>[2x]GSHMRSRRVDVMDVMNRLILAMDLMNRDDALRVTGEVREYIDTVKIGYPLVLSEGMDIIAEFRKRFGCRIIADFAVADIPETNEKICRATFKAGADAIIVHGFPGADSVRACLNVAEEMGREVFLLTEMSHPGAEMFIQGAADEIARMGVDLGVKNYVGPSTRPERLSRLREIIGQDSFLISPGVGAQGG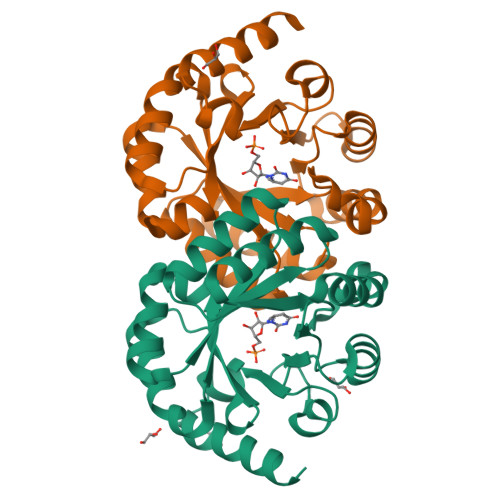DPGETLRFADAIIVGRSIYLADNPAAAAAGIIESIKDLRIPEDPAANKARKEAELAAATAEQ> STGGVSPAATSAPLDWTTFRRVFLIDDAWRPLMEPELANPLTAHLLAEYNRRCQTEEVLPPREDVFSWTRYCTPDEVRVVIIGQDPYHHPGQAHGLAFSVRANVPPPPSLRNVLAAVKNCYPEARMSGHGCLEKWARDGVLLLNTTLTVKRGAAASHSRIGWDRFVGGVIRRLAARRPGLVFMLWGTHAQNAIRPDPRVHCVLKFSHPSPL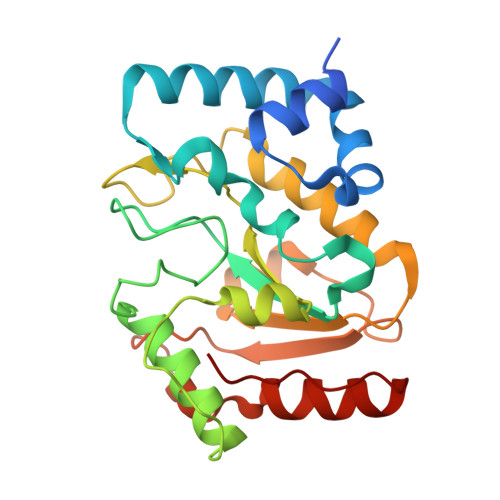SKVPFGTCQHFLVANRYLETRSISPIDWSV> HHHHHHHENLYFQGLEEGFLEDSRASLALRNFYMNRDFRDGAGRAKSEEWAQGFLFDYRSGYTEGTLGVGLDLLGKLGVRLDSGAGRSGTGLLPLRDDGSAAGDYARLDATAKLRLSRSELKVGGLVPKLPTIQPNYGRLFPQVFQGALLTSGELSGLSLNLGRLT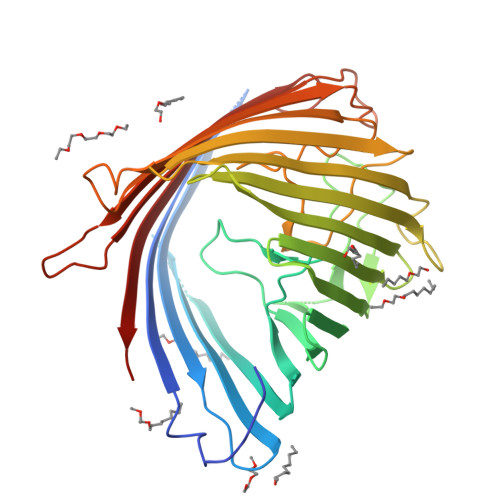EVSQRNEAGTSDLALFNRNRRFAGAAQADRFDLAGLDYRIAPDWTGSYHYGELEQVYAQHFLGLKGRIGIAADSLESDLRLALSRDTGGARGGRIDNRSFSGSLTYRLRNGQAFGLGYQRMSGDHGFPYLEGTDPYLVNFGQYNDFAEAGESSWQLRYDCDFAPLGVPGLSLMTRYFSGHGAKPKGADGSREWERDSDLRYVLQGGALKGLGLVWRNATYRSAFSRDIDENRLYLTYELPLF> MVKLRDWQEKLKDKVIEGLRNNFLVALNAPTGSGKTLFSLLVSLEVKPKVLFVVRTHNEFYPIYRDLTKIREKRNITFSFLVGKPSSCLYAEKGAESEDIPCKYCELKGSIVEVKTDDSPLSLVKKLKKDGLQDKFCPYYSLLNSLYKADVIALTYPYFFIDRYREFIDIDLREYMIVIDEAHNLDKVNELEERSLSEITIQMAIKQSKSEESRRILSKLLNQLREVVLPDEKYIKVENVPKLSKEELEILADDYEDIRKDSLKQGKVNKIHIGSILRFFSLLSIGSFIPFSYSKRLVIKNPEISYYLNLLNDNELSIILMSGTLPPREYMEKVWGIKRNMLYLDVEREIQKRVSGSYECYIGVDVTSKYDMRSDNMWKRYADYLLKIYFQAKANVLVVFPSYEIMDRVMSRISLPKYVESEDSSVEDLYSAISANNKVLIGSVGKGKLAEGIELRNNDRSLISDVVIVGIPYPPPDDYLKILAQRVSLKMNRENEEFLFKIPALVTIKQAIGRAIRDVNDKCNVWLLDKRFESLYWKKNLKCLNANKMKL

XPD (xeroderma pigmentosum group D) is a 5′-3′ superfamily 2 (SF2) helicase that unwinds damaged DNA during the process of nucleotide excision repair (NER). The major enzymatic function of XPD is to unwind the DNA double helix around lesions such as photoproducts to allow repair. In eukaryotes, XPD is one of the components of transcription factor IIH (TFIIH) along with nine other protein subunits. The mechanism of XPD helicase activity remains unclear with uncertainties about the binding of the 3′-end of the translocated DNA strand, the positioning of the junction between single- and double-stranded DNA and the role of protein conformational change in unwinding the DNA.

The crystal structure of SaXPD, obtained from crystals that grew after an unexpectedly long (3 months) time, revealed the absence of the HD2 domain, which most probably was proteolytically cleaved. Interestingly, the rest of the domains maintained the closed conformation, with the Arch domain being only slightly shifted compared to the full-length protein, probably due to lost interactions between the Arch domain and HD2 domain. The crystal packing positioned the Arch domain from a symmetric molecule in place of the missing HD2 domain. Remarkably the structure of SaXPD with HD2 missing adopts the same closed state as the full-length protein, consistent with its stability, recently highlighted by spin labelling and mutational analysis of residues at this interface in TaXPD. In contrast, the integrity of the FeS cluster/domain is greatly affected when not stabilized by the contact with the Arch domain. Overall, the data indicate a highly stable closed conformation of the pore. However, in the case of Sulfolobus acidocaldarius XPD (SaXPD) the ‘pore’ does not actually exist when the molecule is viewed as a surface, rather a pore appears only in cartoon representations.3-[[N-[4-METHYL-PIPERAZINYL]CARBONYL]-PHENYLALANINYL-AMINO]-5-PHENYL-PENTANE-1-SULFONIC 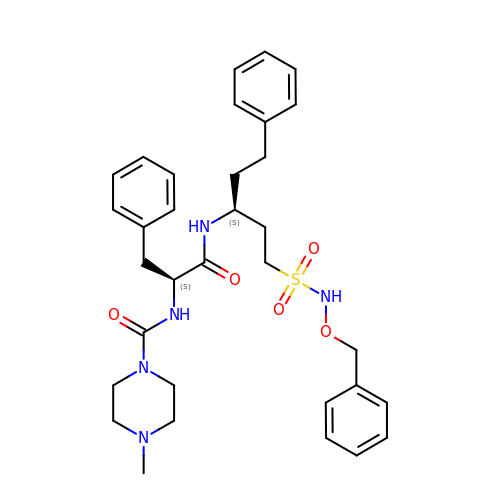ACID BENZYLOXY-AMIDE | C33 H43 N5 O5 S | PPIYQXGSPPWVLJ-CONSDPRKSA-N(2S)-2-[[(2S)-2-[2-[(2-azanyl-4-oxidanylidene-3H-pteridin-7-yl)carbonylamino]ethanoylamino]-3-phenyl-propanoyl]amino]-5-(phenylmethoxycarbonylamino)pentanoic acid | C31 H33 N9 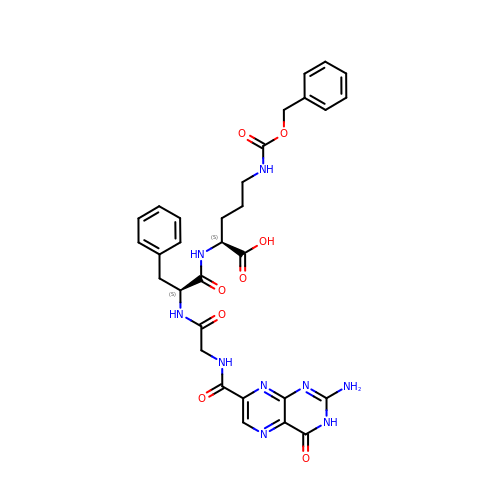O8 | QOJLCYQYXRRJPT-SFTDATJTSA-N>MATLQDIGVSAGINILSAFVFFIIFAVLRLQPFNDRVYFSKWYLKGLRSSPARGGAFAQRFVNLDFRSYMKFLNWMPEALKMPEPELIDHAGLDSVVYLRIYWLGLKIFTPIAVLAWAVLVPVNWTNNTLEMAKQLRNVTSSDIDKLSVSNIPEYSMRFWTHIVMAYAFTIWTCYVLMKEYETIANMRLQFVASEARRPDQFTVLVRNVPPDADESVSELVEHFFLVNHPDHYLTHQVVCNANKLADLVKKKKKLQNWLDYYQLKYARNNSQRIMVKLGFLGLWGQKVDAIEHYIAEIDKISKEISKEREEVVNDPKAIMPAAFVSFKTRWAAAVCAQTQQTRNPTQWLTEWAPEPRDVFWSNLAIPYVSLTVRRLIMHVAFFFLTFFFIVPIAFVQSLATIEGIVKAAPFLKFIVDDKFMKSVIQGFLPGIALKLFLAFLPSILMIMSKFEGFTSISSLERRAAFRYYIFNLVNVFLASVIAGAAFEQLNSFLNQSANQIPKTIGVAIPMKATFFITYIMVDGWAGVAGEILMLKPLIMFHLKNAFLVKTDKDREEAMDPGSIGFNTGEPRIQLYFLLGLVYAPVTPMLLPFILVFFALAYIVYRHQIINVYNQEYESAAAFWPDVHGRVIAALVISQLLLMGLLGTKHAALAAPFLIALPVLTIGFHHFCKGRYEPAFIRYPLQEAMMKDTLETAREPNLNLKGYLQNAYVHPVFKGDEDDYDIDDKLGKFEDEAIIVPTKRQSRRNTPAPSII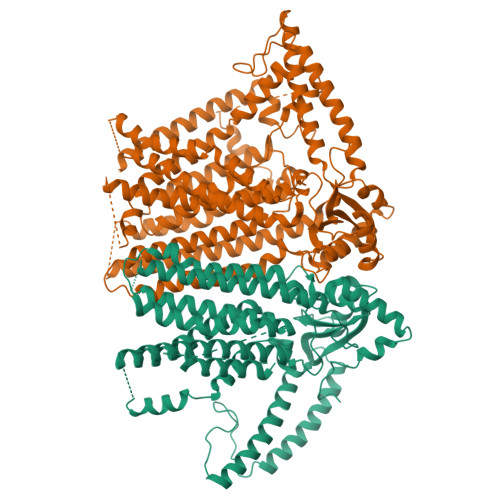SGDDSPSLPFSGKLVSNSLE[2x]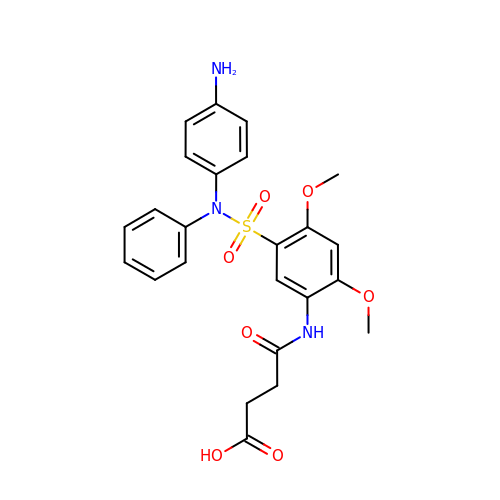4-({5-[(4-aminophenyl)(phenyl)sulfamoyl]-2,4-dimethoxyphenyl}amino)-4-oxobutanoic acid | C24 H25 N3 O7 S | LOWPPNMRMWEKTJ-UHFFFAOYSA-N>MRGSHHHHHHGSMASKVESRQAAVLAIATANPPNIFYQADYPDFYFRVTKSEHMTQLKDKFKRMCEKSMIRKRHMYLTEDVIKENPNIGILNAPSFNARQEIMVEEVPKLGKEAALKAIKEWGQPLSKLTHLIFCTSSGVNMPSADYHLAKIMGLPPYVQRTMIYQQGCFAGATALRLAKDIAENNGGHTRILIVCVELMVVCFQAPSDTYLDLLVGNAIFSDGAAAAIVGADLDTTTERPIFNIVSANQTTIPDSEDGIVGHIREMGMKYYLSRTVPQVIGNNIVQCCRDTFTPLGINDWNSMFYIVHPGGPAVLRMMEEKLGLSKERMRASWHVL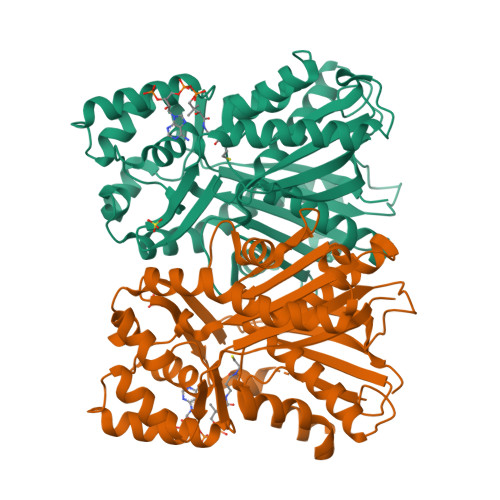SEYGNMWGPSVLFILDEMRNKSMEEGKSTTGEGLEWGVMFGFGPGLTVETVVLRSVAIN[4x]>MKFKHQGLVADLLPNIRVMQGVGHFMFNYYSEGKKFPHRIYCIVTLLLLLLQYGMMAVNLMMESDDVDDLTANTITMLFFLHPIVKMIYFPVRSKIFYKTLAIWNNPNSHPLFAESNARFHALAITKMRRLLFCVAGATIFSVISWTGITFIEDSVKRITDPETNETTIIPIPRLMIRTFYPFNAMSGAGHVFALIYQFYYLVISMAVSNSLDVLFCSWLLFACEQLQHLKAIMKPLMELSATLDTVVPNSGELFKAGSADHLRESQGVQPSGNGDNVLDVDLRGIYSNRQDFTATFRPTAGTTFNGGVGPNGLTKKQEMLVRSAIKYWVERHKHVVRLVTAVGDAYGVALLLHMLTTTITLTLLAYQATKVNGVNVYAATVIGYLLYTLGQVFLFCIFGNRLIEESSSVMEAAYSCHWYDGSEEAKTFVQIVCQQCQKAMSISGAKFFTVSLDLFASVLGAVVTYFMVLVQLK[3x];> MASILDCPIVSVNARVWRFWSFVLKHDAMRYISIIPVTVMTFFMFTDLCRSWGNIQELIIKAYFAVLYFNAVLRTLILVKDRKLYENFMQGISNVYFEISHIDDHKIQSLLKSYTVRARMLSISNLALGAIISTCFVVYPIFTGERGLPYGMFIPGLDSFRSPHYEIIYIVQVVLTFPGCCMYIPFTSFFASTTLFGLVQIKTLQRQLQTFKDNINSQDKEKVKAKVVKLIEDHKRIITYVSELNSLVTYICFVEFLSFGMMLCALLFLLNVIENHAQIVIVAAYIFMIISQIFAFYWHANEVREESMNLAEAAYSGPWVELDNSIKKKLLLIILRAQQPLEITVGNVYPMTLEMFQSLLNASYSYFTLLRRVYN

Most insects, including human-targeting mosquitoes, detect odors through odorant-activated ion channel complexes consisting of a divergent odorant-binding subunit (OR) and a conserved co-receptor subunit (Orco). As a basis for understanding how odorants activate these heteromeric receptors, we report here cryo-EM structures of two different heteromeric odorant receptor complexes containing ORs from disease-vector mosquitos Aedes aegypti or Anopheles gambiae. We determined the structure of a heteromeric complex formed by ORs from these species in complex with a Apocrypta bakeri fig wasp Orco that is amenable to structural determination. We find that these complexes form asymmetric tetramers containing 1 OR and 3 Orco subunits, where activation of the sole OR subunit upon ligand binding suffices to open the ion conduction pathway.

We first focused on the conserved OR10 receptor family, which detects indole and derivatives in various mosquito species. The cryo-EM structure of an OR/Orco complex has a 1:3 subunit stoichiometry. Aside from the different extracellular loops, the OR10 and Orco subunits have very similar fold, despite having only 15.1% sequence identity. Importantly, the residues in Orco that are in direct contact with AaOR10 in our structure exhibit 97% sequence identity and 100% sequence similarity to those in Ae. aegypti Orco, providing a structural explanation to the ability of Orcos to substitute for each other. The cryo-EM dataset of the unbound AaOR10/Orco complex contained two distinct subsets of particles. The existence of active and inactive states in the unbound dataset suggests that even in the absence of odorant, AaOR10/Orco is an equilibrium mixture, consistent with the well-characterized high baseline activity of insect odorant receptors in the absence of odorant ligands. The strength and shape of this unmodeled density suggest that it represents a lipid molecule co-purified with the heteromeric complex. The long tail of this density, in turn, is wedged into the groove between the S3-S6 and extends into the transmembrane space, helping stabilize the inactive conformation by preventing helix S6 from moving towards helix S3. Thus, both the presumptive lipid and the phenyl ring of Phe136 appear to stabilize the inactive conformation of AaOR10/Orco complex by holding S6 in place.>ADSDINIKTGTTDIGSNTTVKTGDLVTYDKENGMAKKVFYSF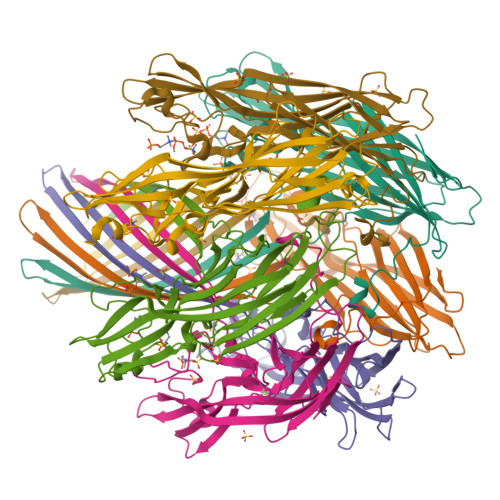IDDKNHNKKLLVIRTKGTIAGQYRVYSEEGANKSGLAWPSAFKVQLQLPDNEVAQISDYYPRNSIDTKEYMSTLTYGFNGNVTGDDTGKIGGLIGANVSIGHTLKYVQPDFKTILESPTDKKVGWKVIFNNMVNQNWGPYDRDSWNPVYGNQLFMKTRNGSMKAADNFLDPNKASSLLSSGFSPDFATVITMDRKASKQQTNIDVIYERVRDDYQLHWTSTNWKGTNTKDKWTDRSSERYKIDWEKEEMTN[7x]>[6x]DTGCAVSWSGKELKCGSGIFVIDNVHT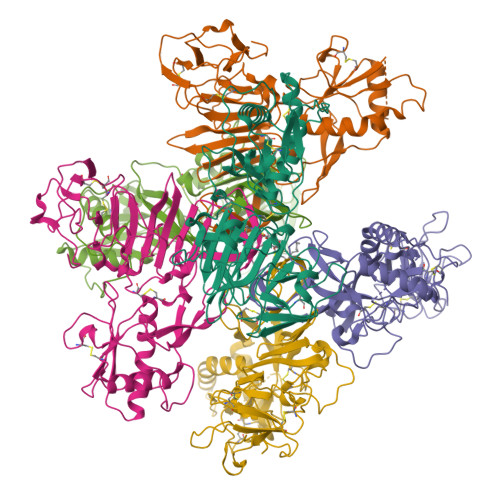WTEQYKFQPESPARLASAILNAHEDGVCGIRSTTRLENIMWKQITNELNYVLWEGGHDLTVVAGDVKGVLSKGKRALAPPVNDLKYSWKTWGKAKIFTPEAKNSTFLIDGPDTSECPNERRAWNFLEVEDYGFGMFTTNIWMKFREGSSEVCDHRLMSAAIKDQKAVHADMGYWIESSKNQTWQIEKASLIEVKTCLWPKTHTLWSNGVLESQMLIPKAYAGPFSQHNYRQGYATQTVGPWHLGKLEIDFGECPGTTVTIQEDCDHRGPSLRTTTASGKLVTQWCCRSCTMPPLRFLGEDGCWYGMEIRPLSEKEENMVKSQVSAHHHHHH> MGSSHHHHHHSQDPNSMPDNTIQWDKDADGIVTLTMDDPSGSTNVMNEAYIESMGKAVDRLVAEKDSITGVVVASAKKTFFAGGDVKTMIQARPEDAGDVFNTVETIKRQLRTL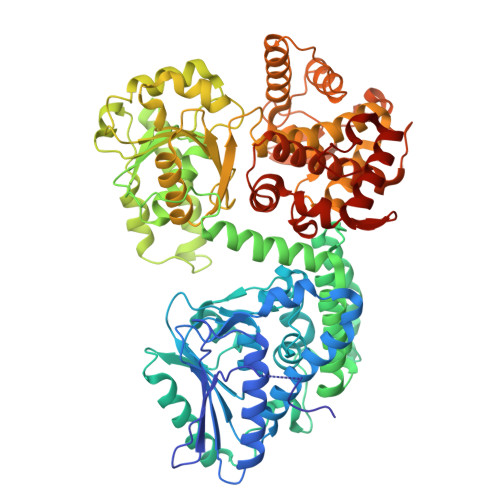ETLGKPVVAAINGAALGGGLEIALACHHRIAADVKGSQLGLPAVTLGLLPGGGGVTRTVRMFGIQNAFVSVLAQGTRFKPAKAKEIGLVDELVATVEELVPAAKAWIKEELKANPDGAGVQPWDKKGYKMPGGTPSSPGLAAILPSFPSNLRKQLKGAPMPAPRAILAAAVEGAQVDFDTASRIESRYFASLVTGQVAKNMMQAFFFDLQAINAGGSRPEGIGKTPIKRIGVLGAGMMGAGIAYVSAKAGYEVVLKDVSLEAAAKGKGYSEKLEAKALERGRTTQERSDALLARITPTADAADFKGVDFVIEAVFENQELKHKVFGEIEDIVEPNAILGSNTSTLPITGLATGVKRQEDFIGIHFFSPVDKMPLVEIIKGEKTSDEALARVFDYTLAIGKTPIVVNDSRGFFTSRVIGTFVNEALAMLGEGVEPASIEQAGSQAGYPAPPLQLSDELNLELMHKIAVATRKGVEDAGGTYQPHPAEAVVEKMIELGRSGRLKGAGFYEYADGKRSGLWPGLRETFKSGSSQPPLQDMIDRMLFAEALETQKCLDEGVLTSTADANIGSIMGIGFPPWTGGSAQFIVGYSGPAGTGKAAFVARARELAAAYGDRFLPPESLLS>TGHNTTVFQGVAGQSLQVSCPYDSMKHWGRRKAWCRQLGEKGPCQRVVSTHNLWLLSFLRRWNGSTAITDDTLGG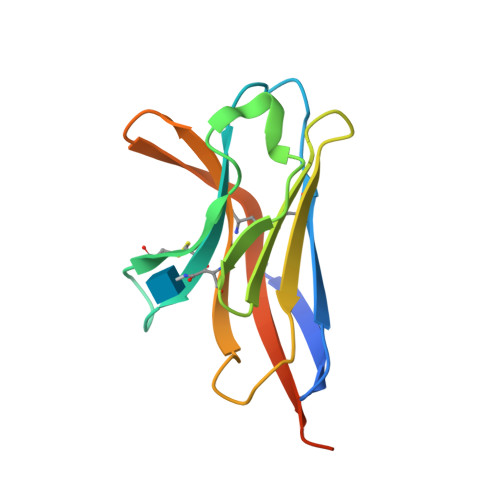TLTITLRNLQPHDAGLYQCQSLHGSEADTLRKVLVEVLADPLGTKHHHHHH[2x]> MAHHHHHHSSGLEVLFQGPNEFETLELEHLLWVNITQVKHSIERAWTRELKSLNLSTEKFAILHELMCLGGESTPHTLARRIVFEPHSVSAIVSRME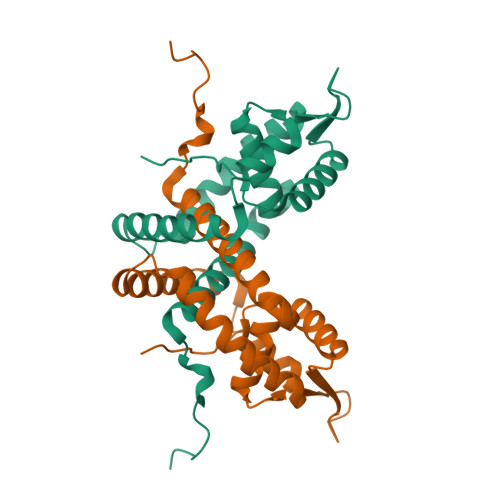KDGLIIKTKDLDKKHMVRIKLSEKAIDTFYQALEISNRVYKQMMASITREEKVELSKTLTKLRNHTLPLTHKHTKTLTPFKYI> VTEEQVHHIVKQALQRYSEDRIGLADYALESGGASVISTRCSETYETKTALLSLF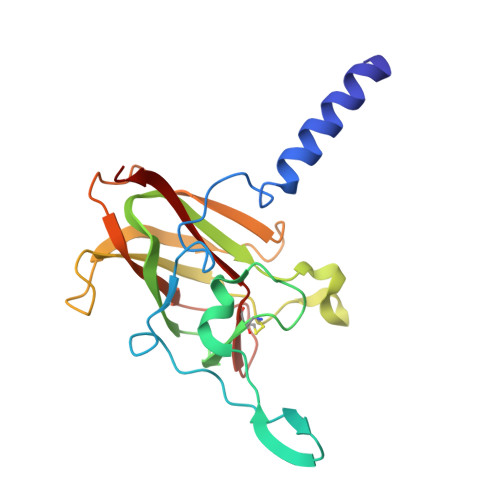GIPLWYHSQSPRVILQPDVHPGNCWAFQGPQGFAVVRLSARIRPTAVTLEHVPKALSPNSTISSAPKDFAIFGFDEDLQQEGTLLGKFTYDQDGEPIQTFHFQAPTMATYQVVELRILTNWGHPEYTCIYRFRVHGEPAH> MGSHHHHHHGSLSKFKRNKHQQHLAQLPKISQSVDDVDFFYAPADFRETLLEKIASAKQRICIVALYLEQDDGGKGILNALYEAKRQRPELDVRVLVDWHRAQRGRIGAAASNTNADWYCRMAQENPGVDVPVYGVPINTREALGVLHFKGFIIDDSVLYSGASLNDVYLHQHDKYRYDRYHLIRNRKMSDIMFEWVTQNIMNGRGVNRLDDVNRPKSPEIKNDIRLFRQELRDAAYHFQGDADNDQLSVTPLVGLGKSSLLNKTIFHLMPCAEQKLTICTPYFNLPAILVRNIIQLLREGKKVEIIVGDKTANDFYIPEDEPFKIIGALPYLYEINLRRFLSRLQYYVNTD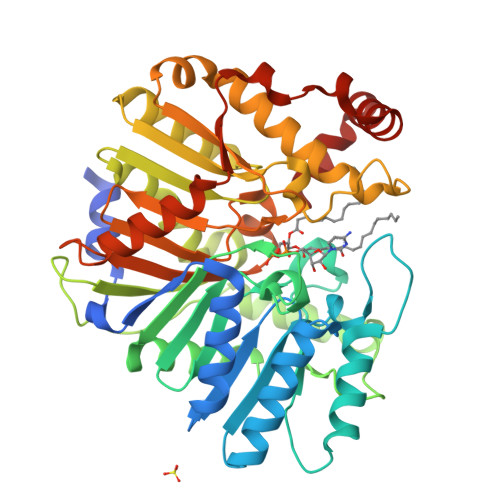QLVVRLWKDDDNTYALKGMWVDDKWMLITGNNLNPRAWRLDLENAILIHDPQLELAPQREKELELIREHTTIVKHYRDLQSIADYPVKVRKLIRRLRRIRIDRLISRIL> GRRTVPRGTLRKIIKKHKPHLRLAANTDLLVHLSFLLF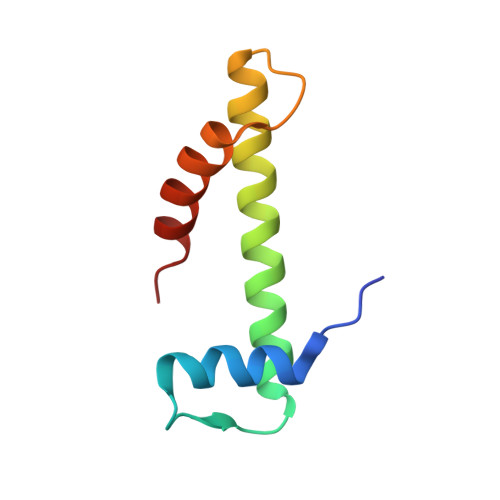LHRLAEEARTNAFENKCKIIKPEHTIAAAKVILKKSRG> HPETLVKVKDAEDQLGARVGYIELDL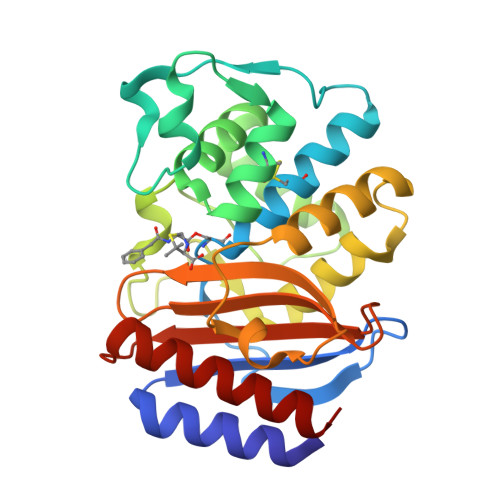NSGKILESFRPEERFPMMSTFKVLLCGAVLSRVDAGQEQLGRRIHYSQNDLVEYSPVTEKHLTDGMTVRELCSAAITMSDNTAANLLLTTIGGPKELTAFLHNMGDHVTRLDRWNPELNEAIPNDERDTTMPAAMATTLRKLLTGELLTLASRQQLIDWMEADKVAGPLLRSALPAGWFIADKSGAGERGSRGIIAALGPDGKPSRIVVIYTTGSQATMDERNRQIAEIGASLIKHW4-azanyl-6-[1,2,2-tris(chloranyl)ethenyl]benzene-1,3-disulfonamide | C8 H8 Cl3 N3 O4 S2 | 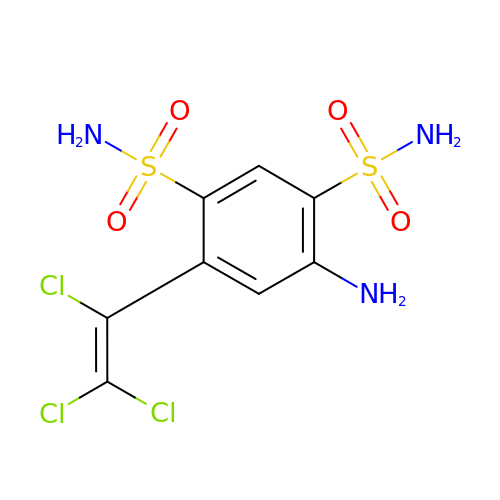QOVTVIYTBRHADL-UHFFFAOYSA-N(4~{S})-7,8-bis(chloranyl)-9-methyl-1-oxidanylidene-spiro[2,4-dihydropyrido[3,4-b]indole-3,4'-piperidine]-4-carbonitrile 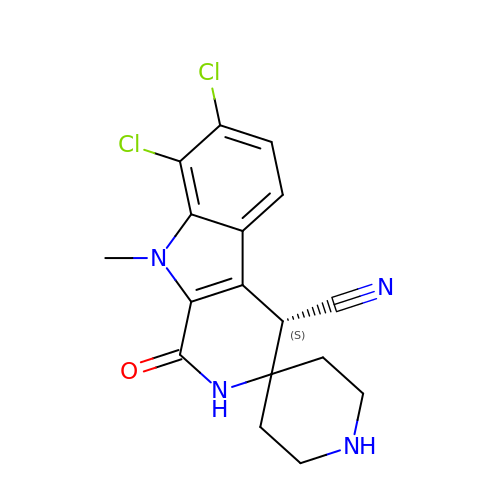| C17 H16 Cl2 N4 O | OWAWOKKHZNRHGV-JTQLQIEISA-N>[4x]MSTPDALGSDAARAARAAALLRAAANDLKRNDRAAEADLGLPPGSFGDYVSGRLPITWDLISRAAQAWPLNERDLLPI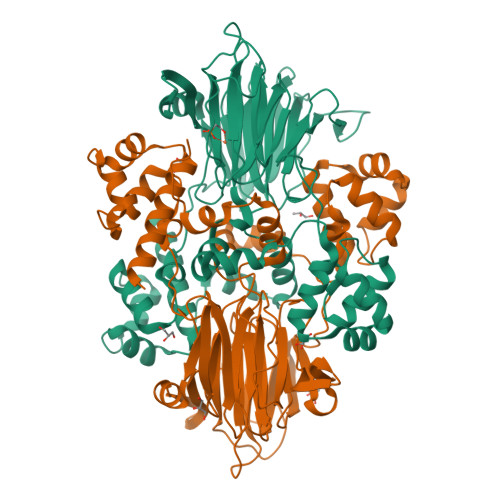HNDTPQGLRMMRVKESEASSRIIERGGGPYYEYRDTAMSRQASYRPEWISMLRVVEDDDPDNPLVEWNKGHLLYQFTYFVGPVNYYFRSGGRSHCVPMNTGDSVWGLPFAPHSFTARSADEPAYILALTYGGELTGDAQRELATFGRAVTSSLALTPGDHGAMLRSVMAARLTTVTELADRSGLKTDRVAALCRTPARAEWPELSALAEALGVSVRELLVPHTTTEADVRIQPGRTASRWSYPGPDAPAYRFTQLAGDPLHPHTTSLAVDVLTARPDAPLPPTYQHQYLYVLGEQPVSVRWRYNGEQYDGRLEPGDSAYVIPGIEFSLSAEKPTELLMLRIGGSATPDVRFALGAMPDGAIGRYIAEDRLWY>[2x]TKDNLTGDIVIIGAGAAGSLLAHYLARFSNMKIILLEAGHSHFNDPVVTDPMGFFGKYNPPNENISMSQNPSYSWQGAQEPNTGAYGNRPIIAHGMGFGGSTMINRLNLVVGGRTVFDNDWPVGWKYDDVKNYFRRVLVDINPVRDNTKASITSVALDALRIIAEQQIASGEPVDFLLNKATGNVPNVEKTTPDAVPLNLNDYEGVNSVVAFSSFYMGVNQLSDGNYIRKYAGNTYLNRNYVDENGRGIGKFSGLRVVSDAVVDRIIFKGNRAVGVNYIDREGIMHYVKVNKEVVVTSGAFYTPTILQRSGIGDFTYLSSIGVKNLVYNNPLVGTGLKNHYSPVTITRVHGEPSEVSRFLSNMAANPTNMGFKGLAELGFHRLDPNKPANANTVTYRKYQLMMTAGVGIPAEQQYLSGLSPSSNNLFTLIADDIRFAPEGYIKIGTPNIPRDVPKIFFNTFVTYT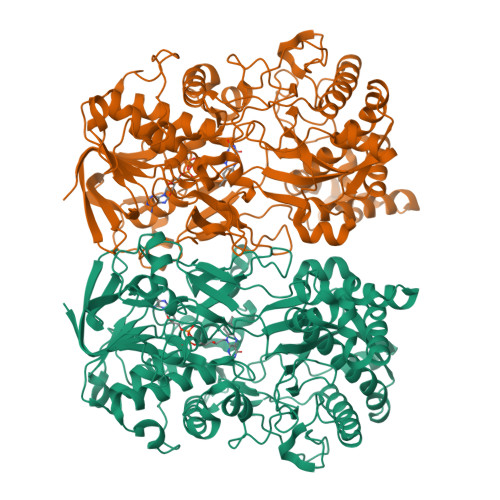PTSAPADQQWPIAQKTLAPLISALLGYDIIYQTLMSMNQTARDSGFQVSLEMVYPLNDLIYKLHNGLATYGANWWHYFVPTLVGDDTPAGREFADTLSKLSYYPRVGAHLDSHQGCSCSIGRTVDSNLKVIGTQNVRVADLSAAAFPPGGNTWATASMIGARAVDLILGFPYLRDLPVNDVPILNVN>[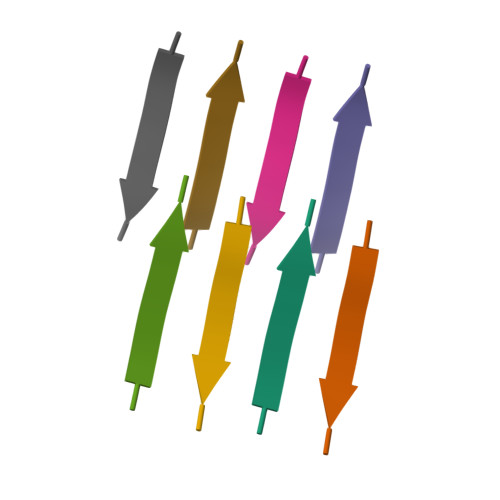4x]MVGGVV> GPLGSPEFPGRPAFEGLVQRIRLIVPSTLRGGDGEAGPYSPSSLPSRCAFQFHGHDGSDESFPIEYVLRLMNDWAEVPCNPYLRIQNTGVSVLFQGFFHRPHNAPGGAITPERTNVILGSTETTGLSLGDLDTIKGRL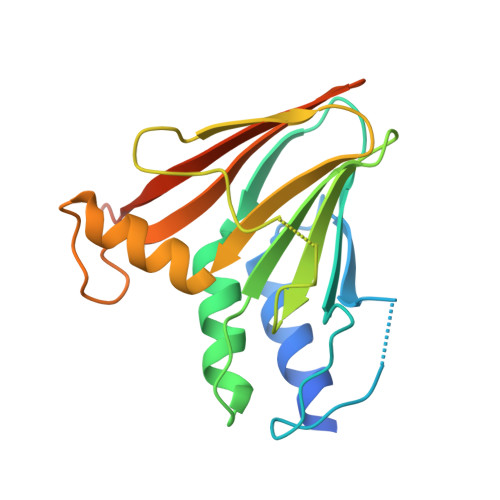GLDARPMMASMWISCFVRMPRVQLAFRFMGPEDAGRTRRILCRAA>GSDFSQKPIRYTVATRVGKPYFSWREEPEGVHYEGNERFEGYAVDLIYMLAQECKFDFNFEPVRDNKYGSYDANTDEWDGIIRQLIDNNAQIGICDLTITQARRSVVDFTVPFMQLGISILSYKGTDIGSLHDLVDQNKVQFGTIRGGATSVYFSESNDTDNRMAWNKMLSFKPDAFTKNNEEGVDRVKLS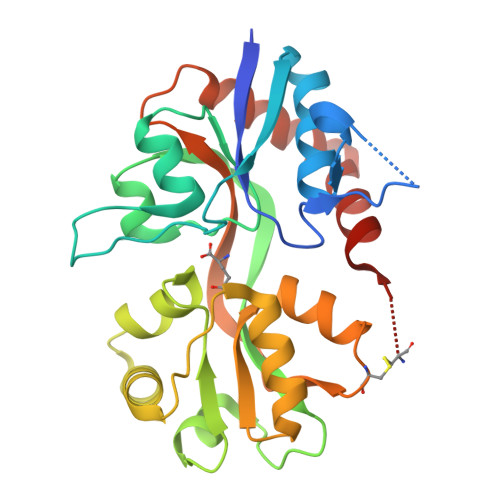KGTYAFLMETTNLQYYVQRNCELTQIGESFGEKHYGIAVPLNADFRSNLSVGILRLSERGELFKLRNKWFNSNESTCD[2x]>[26x]MARKRTSKNDPLRMYLNYVRKLQTMGDAYDESAKYRIANFENGFKSLHMVENEFKQYLANVIDEAIKSGASPQDLPYVNEIKLALMKIFTSWLKYSNEKLGANEIAINV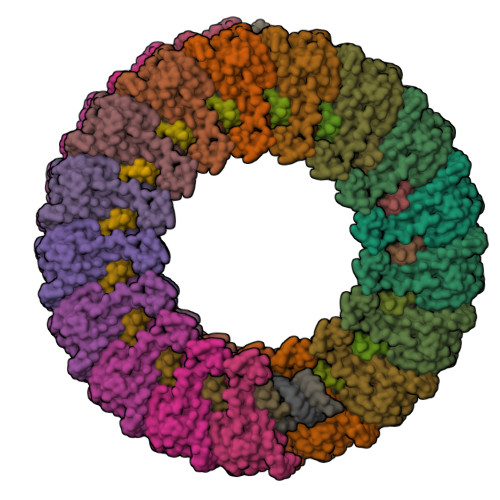AGTATMTLTENLYGTRVSCEEAVSLINSIFAVWVGVEPFEAEEREGACLVTPRSPLPPVPISSPTGFSAPIQEVLQAKSPEEIIGVKGGA;>MPSRRTGITTEDAITKYSVKAKTEQTAYKNATKDMVVQAQNIMNFYSVVNQALIPWLNAHGVGGNLRILYRQLANEYVKVLNTKQSGEVIKRLKIALRHKYWLRGLDEAMLDEFMDYIDSLKSTTTNYIIFNMQSSK[26x]5,6-dihydroxy-2-[(2-phenyl-1H-indol-3-yl)methyl]pyrimidine-4-carboxylic 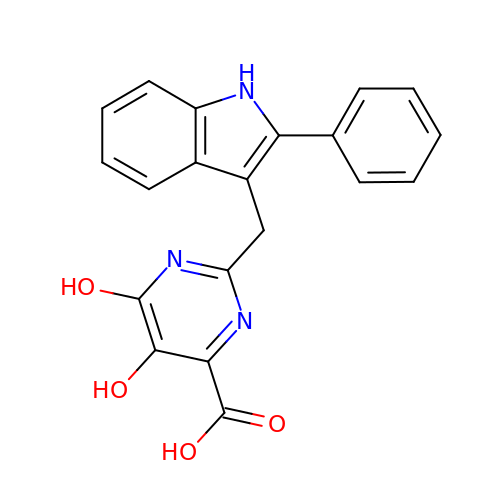acid | C20 H15 N3 O4 | JONQCFJPPWOWOJ-UHFFFAOYSA-N>[6x]MGHHHHHHQQLASFLSGTWQSGRGRSRLIHHAISGEALWEVTSEGLDMAAARQFAIEKGAPALRAMTFIERAAMLKAVAKHLLSEKERFYALSAQTGATRADSWVDIEGGIGTLFTYASLGSRELPDDTLWPEDELIPLSKEGGFAARHLLTSKSGVAVHINAFNFPCWGMLEKLAPTWLGGMPAIIKPATATAQLTQAMVKSIVDSGLVPEGAISLICGSAGDLLDHLDSQDVVTFTGSAATGQMLRVQPNIVAKSIPFTMEADSLNCCVLGEDVTPDQPEFALFIREVVREMTTKAGQKCTAIRRIIVPQALVNAVSDALVARLQKVVVGDPAQEGVKMGALVNAEQRADVQEKV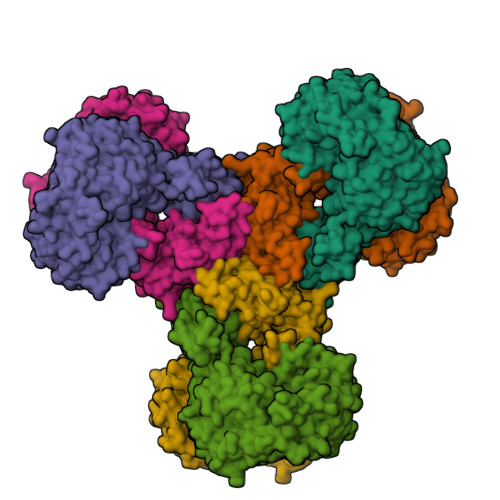NILLAAGCEIRLGGQADLSAAGAFFPPTLLYCPQPDETPAVHATEAFGPVATLMPAQNQRHALQLACAGGGSLAGTLVTADPQIARQFIADAARTHGRIQILNEESAKESTGHGSPLPQLVHGGPGRAGGGEELGGLRAVKHYMQRTAVQGSPTMLAAISKQWVRGAKVEEDRIHPFRKYFEELQPGDSLLTPRRTMTEADIVNFACLSGDHFYAHMDKIAAAESIFGERVVHGYFVLSAAAGLFVDAGVGPVIANYGLESLRFIEPVKPGDTIQVRLTCKRKTLKKQRSAEEKPTGVVEWAVEVFNQHQTPVALYSILTLVARQHGDFVD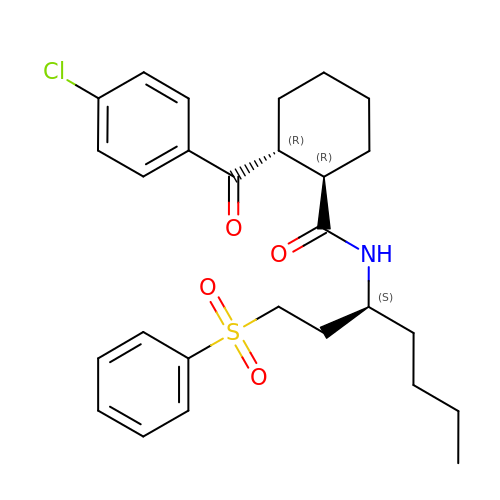(1R,2R)-2-[(4-chlorophenyl)carbonyl]-N-{(1S)-1-[2-(phenylsulfonyl)ethyl]pentyl}cyclohexanecarboxamide | C27 H34 Cl N O4 S | GOPKEHWOLDXUST-ICDZXHCJSA-N> MDPVLGDVIATRIYKACFKHVYGKNMKAYSEKDEAKFDQCLTSYVESYKS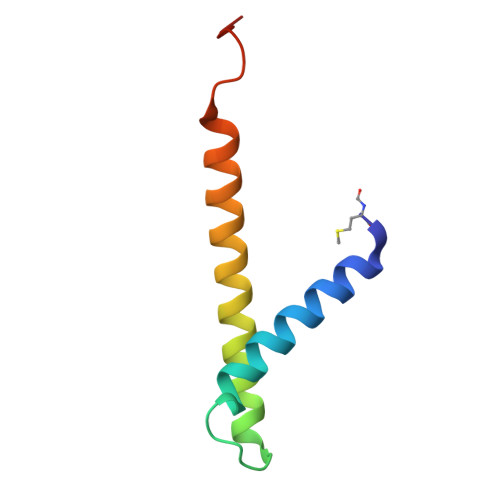VTNHFITYLGQLPKKGLSLDGS5-[(4,6-dimethoxypyrimidin-2-yl)carbamoylsulfamoyl]-1-methyl-pyrazole-4-carboxylic acid | C12 H14 N6 O7 S | 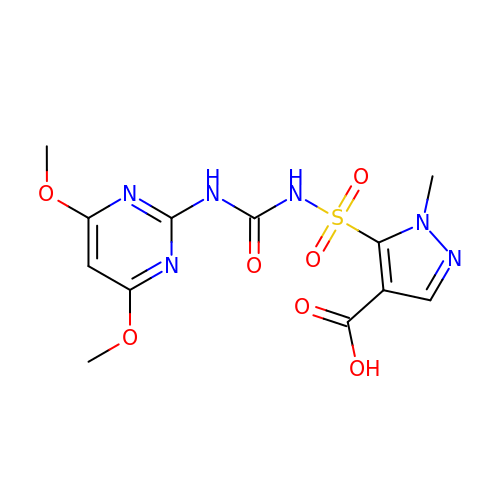VXMNDQDDWDDKOQ-UHFFFAOYSA-N>MELFQTADWKKQKHVPVIEVLRAEGGVVEVKVSVGKEIPHPNTTEHHIAWIELVFQPEGSKFPYVVGRAEFAAHGASVDGPNTSGVYTDPVAVFAFKAEKSGKLTAFSYCNIHGLW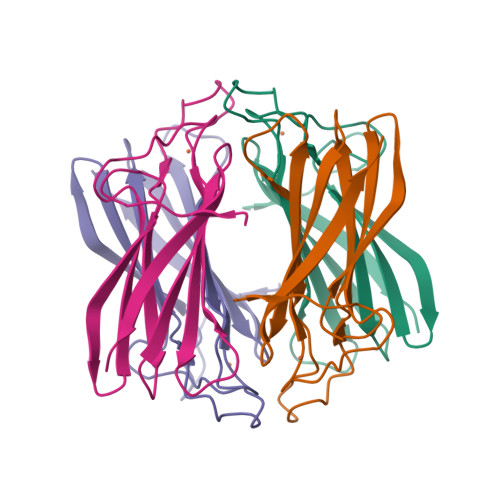MGEATLSLE[16x]> APDSIDYRKKGYVTPVKNQGQCGSCWAFSSVGALEGQLKKATGALLNLAPQNLVDCVSENDGCGGGYMTNAFQYVQRNRGIDSEDAYPYVGQDESCMY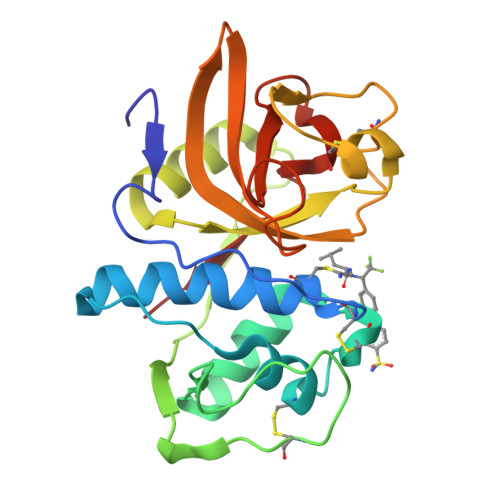NPTGKAAKCRGYREIPEGNEAALKRAVAAVGPVSVAIDASLTSFQFYSAGVYYDENCSSDALNHAVLAVGYGIQAGNKHWIIKNSWGESWGNAGYILMARNKNNACGIANLASFPKM> MADEEAMLAKVQASW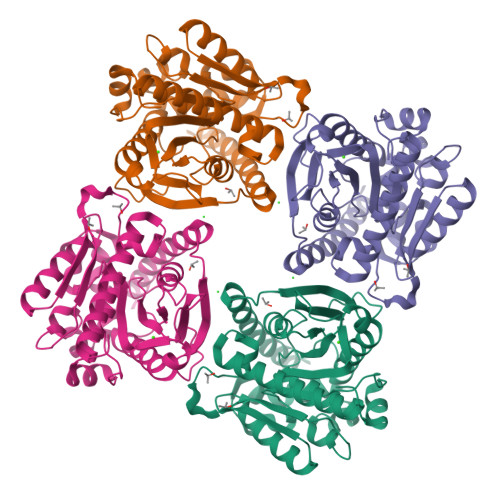AQTAARDKARYADERVPEDVHWETEYRYEQSADPQQTLNLYYPAKRRNATMPTVIDIHGGGWFYGDRNLNRNYCRYLASQGYAVMGMGYRLLPDVDLRGQIQDIFASLRWLSHFGPQRGFDLDHVLLTGDSAGGHLASLVACIQQSAELQELFGVSRVNFNFTLVALVCPVAEPSKLPEAAGDMSDMAAFYLDKLSGGDQALVDHLNFSQVVKGLDLPPFMLIGGQNDSFYLQSQALLKVFDANHVTYTTKLWPASAGPHLKHVFNVQHWEWPESIETNLEMLRTFDALSKQQDQAEENEFE> MIKSALLVLEDGTQFHGRAIGATGSAVGEVVFNTSMTGYQEI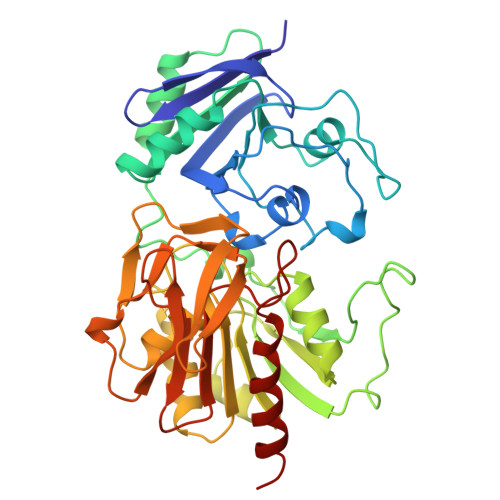LTDPSYSRQIVTLTYPHIGNVGTNDADEESSQVHAQGLVIRDLPLIASNFRNTEDLSSYLKRHNIVAIADIDTRKLTRLLREKGAQNGCIIAGDNPDAALALEKARAFPGLNGMDLAKEVTTAEAYSWTQGSWTLTGGLPQAKKEDELPFHVVAYDFGAKRNILRMLVDRGCRLTIVPAQTSAEDVLKMNPDGIFLSNGPGDPAPCDYAITAIQKFLETDIPVFGICLGHQLLALASGAKTVKMKFGHHGGNHPVKDVEKNVVMITAQNHGFAVDEATLPANLRVTHKSLFDGTLQGIHRTDKPAFSFQGHPEASPGPHDAAPLFDHFIELIEQYRKTAK> MAHATKDLSALARTDEEVLVQGGLTFHDITELVAQHTEKKTPKAWWAAFSVAFLGMLTLVAMLAYQVWNGVGVWGNNIPVGWGWPIVNFVFWVGI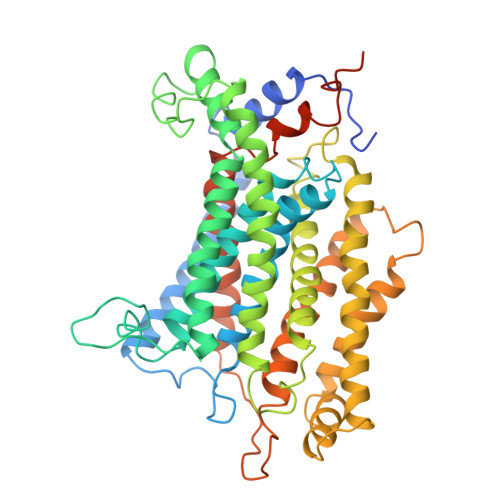GHAGTLISAILFLFRQRWRTSINRAAEAMTIFAVICALIFPTFHVGRVWAIYWTLPIPNQMEMWPQFKSPLLWDVFAVSSYFIVSLVFWYVGLIPDLATLRDRAALMGRRLRAKILGFFALGWCGANRHWRNYEKVYMLLAGLATPLVLSVHSVVSFDFAVSIIPGWHTTIFPPYFVAGAIFSGFAMVVTLMVIARKAYGLENVITIDHLEKMNIIMLVTGTMVGFAYITEFFIAWYSGVPYEQYAFINRATGPYAWAYWTMMSCNLIFPQFFWIKKLRRNIPFMFIASIVVNIGMWFERFVITITSLHRDYLPSSWDYFVPTWVDVLTLIGSFGLFFTLFLLFLRFVPMVAIAEVKGVLPEADPHFYETHGDGHSRPAEVQVNRGRSS>[2x]EAVVISGRKLAQQIKQEVRQEVEEWVASGNKRPHLSVILVGENPASHSYVLNKTRAAAVVGINSETIMKPASISEEELLNLINKLNNDDNVDGLLVQLPLPEHIDERRICNAVSPDKDVDGFHVINVGRMCLDQYSMLPATPWGVWEIIKRTGIPTLGKNVVVAGRSKNVGMPIAMLLHTDGAHERPGGDATVTISHRYTPKEQLKKHTILADIVISAAGIPNLITADMIKEGAAVIDVGINRVHDPVTAKPKLVGDVDFEGVRQKAGYITPVPGGVGPMTVAMLMKNTIIAAKKVLRLEEREVLKSKELGVATN

MTHFD2, a one-carbon metabolism enzyme, is localized in the mitochondria and plays an important role in nucleic acid biosynthesis, amino acid metabolism, and protein synthesis. It is a NAD-dependent enzyme and functions as both 5,10-methylenetetrahydrofolate (CH2-THF) dehydrogenase and 5,10-methenyltetrahydrofolate (CH+-THF) cyclohydrolase, converting CH2-THF to 10-formyl-THF (CHO-THF). MTHFD2 forms a homodimer and each monomer consists of the N-lobe and C-lobe connected by two long α helices. The MTHFD2 gene is upregulated in various cancers but very low or undetectable in normal proliferating cells, and therefore a potential target for cancer treatment.

Superimposition of the MTHFD2/15/21 complex structure on the MTHFD2/NAD+/Pi/21 complex structure reveals that upon the binding of 15, MTHFD2 induces dramatic conformational changes, including the shift of the βe-αE loop in monomer A, destabilization of the αE′-βf′ loop, and movement of the αD2′-αD3′ loop in monomer B. The structure of MTHFD2/NAD+/Pi/21 was obtained by cocrystallization of MTHFD2 with NAD+, phosphate (Pi), and 21. 21 binds to the substrate-binding site while NAD+ is located between the N and C-lobes and surrounded by the βe-αE, βf-αF, βg-αG, and βh-βh1 loops, helix D3, and helix I. Of these secondary structures, the βe-αE loop consists of a G200RSKNVG motif, a conserved fingerprint pattern observed in the Rossmann fold of the MTHFD family. As revealed in the MTHFD2/NAD+/Pi/21 structure, NAD+ is hydrogen bonded to Arg201 and Ser202 on the βe-αE loop. In addition, NAD+ also forms hydrophobic interactions with Thr176 and Val205 and hydrogen-bond interactions with Arg233, Ile276, and Thr316. The phosphate is located in the dimer interface, forming an extensive hydrogen-bond network with Arg201 and Arg233 in monomer A and Asp216′ and His219′ in monomer B. In the presence of NAD+, Arg201 serves as the interaction center to form hydrogen bonds with the phosphate ion, the adenosine ribose ring of NAD+, and also coordinates with Asp216′, His219′, and Asp225′ in monomer B through the salt bridge and hydrogen-bond network. In the MTHFD2/NAD+/Pi/21 structure, Arg233 binds to the phosphate ion and NAD+, providing evidence that Arg233 contributes to the phosphate binding and assists in positioning NAD+. In the absence of 15, the αD2′-αD3′ loop stabilizes the αE′-βf′ loop via an extensive interaction network. Furthermore, in the absence of 15, His219′ in the αE′-βf′ loop binds to phosphate.>MGSSHHHHHHSSGLVPRGSDLQEDEDGVYFSSYGHYGIHEEMLKDKIRTESYRDFIYQNPHIFKDKVVLDVGCGTGILSMFAAKAGAKKVLGVDQSEILYQAMDIIRLN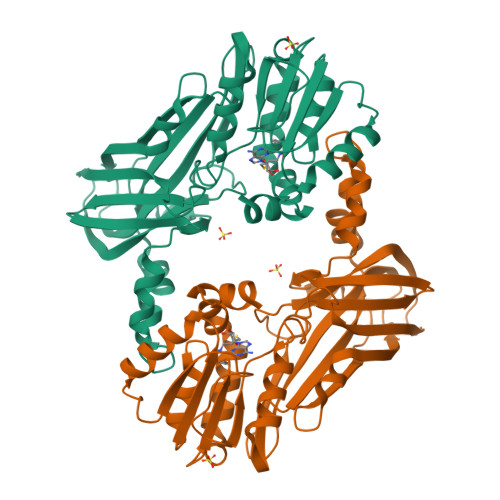KLEDTITLIKGKIEEVHLPVEKVDVIISEWMGYFLLFESMLDSVLYAKNKYLAKGGSVYPDICTISLVAVSDVNKHADRIAFWDDVYGFKMSCMKKAVIPEAVVEVLDPKTLISEPCGIKHIDCHTTSISDLEFSSDFTLKITRTSMCTAIAGYFDIYFEKNCHNRVVFSTGPQSTKTHWKQTVFLLEKPFSVKAGEALKGKVTVHKNKKDPRSLTVTLTLNNSTQTYGLQ[2x]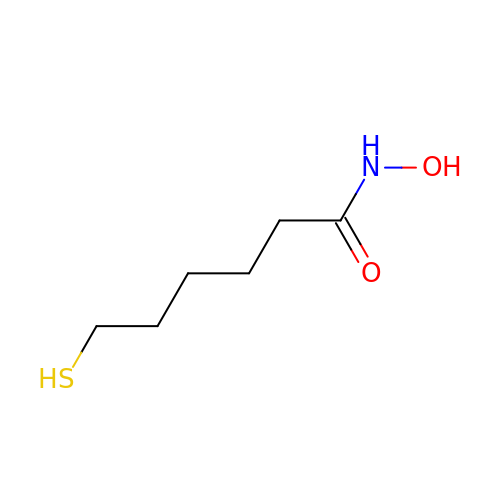N-hydroxy-6-sulfanylhexanamide | C6 H13 N O2 S | UVHGRHBRZBMHBD-UHFFFAOYSA-N>[2x]MKTRITELLKIDYPIFQGGMAWVADGDLAGAVSKAGGLGIIGGGNAPKEVVKANIDKIKSLTDKPFGVNIMLLSPFVEDIVDLVIEEGVKVVTTGAGNPSKYMERFHEAGIIVIPVVPSVALAKRMEKIGADAVIAEGMEAGGHIGKLTTMTLVRQ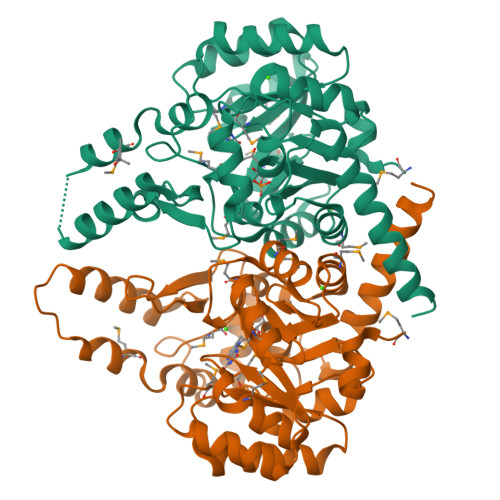VATAISIPVIAAGGIADGEGAAAGFMLGAEAVQVGTRFVVAKESNAHPNYKEKILKARDIDTTISAQHFGHAVRAIKNQLTRDFELAEKDAFKQEDPDLEIFEQMGAGALAKAVVHGDVDGGSVMAGQIAGLVSKEETAEEILKDLYYGAAKKIQEEASRWTGVVRNDLEHHHHHH>MPTPSMEDYLERIYLLIEEKGYARVSDIAEALEVHPSSVTKMVQKLDKSDYLVYERYRGLILTAKGKKIGKRLVYRHDLLEDFLKMIGVDSDHIYEDVEGIEHHLSWDAIDRIG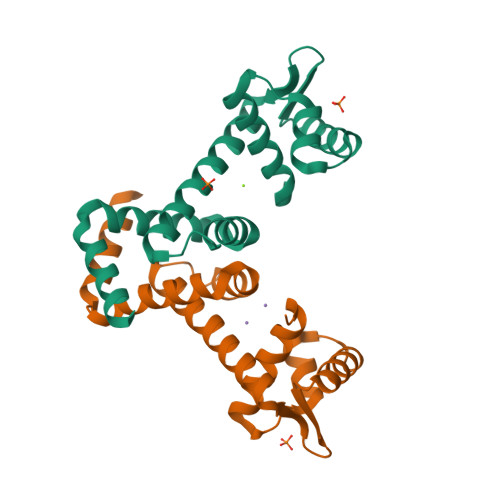DLVQYFQEDPSRLNDLREVQKKNEE[2x]>[2x]MYKTLRLGDRGADVSYLQRQLIAAGARLDIDAIYGSATRDAVMAFQATHGLVADGIAGPKTWSTLSAGRRDPRHLTDADLQRAADRLQVDLAAVRAVNEVESKGAGFLPDGRPVILYERHIMYRQLAAAGLDADALAAKYPALVNSKRGGYAGDAAEYARLASASQISGACALEATSWGAFQIMGFHWKALGYPDVFAFVDAMKVSEAEQLEAFVRFVLADKVMLAALRSKKWAKFAELYNGKAYAENLYDVKLERAFDRYSRAAA

In the present study, we describe a modular endolysin (rare for Gram-negative infecting phages) originating from B. cenocepacia AP3 phage. The structure of endolysin, predicted in silico in BLASTP, is modular, consisting of CBD (10-65 aa; PG_binding_1 domain; pfam01471) at the N-terminus, and DUF3380 domain (pfam11860) at the C-terminus (90-262 aa). Thus, comparable to lysozyme, AP3gp15 cleaves β-1,4-glycosidic bond of PG and releases GlcNAc and MurNAc. Similarly to others, the AP3 endolysin shows a broad spectrum of activity against Gram-negative strains, but no PG-degrading properties with respect to Gram-positives.

The overall structure comprises of two clearly distinguished domains, a smaller N-terminal CBD domain (Lys3 – Ser66), and a larger EAD domain (Asp77 – Ala264) located towards the C-terminus. CBD domain is composed of a bundle of three antiparallel helices (α1-α3) and is joined with EAD via a hinge region spanning amino acids (Ala67 – Thr76). The EAD domain is organized into two sub-domains: first encompassing helices α4-α5 (Asp77 – Glu101) and helices α10 to α15 (Gly185 – Ala266), and the second containing β1 (Ile115 – Tyr117), β2-β3 (Thr176 – Met184) sheet intervened by helices α6 to α9 (Arg119 – Ala175). The structure of the EAD domain of AP3gp15 is characterized by a deep concave cleft at the subdomain interface. Despite a relatively low homology of amino acid sequence (31% and 39% identity, respectively), a high structural homology of the entire AP3gp15 N-terminal part to the domains of clearly identified function strongly suggests its role in PG interaction. The large enzymatic C-terminal domain of AP3 endolysin shows structural homology to proteins of lysozyme family. The comparison to HEWL, the closest structural homologue among lysozymes, allowed to define the core structure of AP3 endolysin, where the entire fold of HEWL is encompassed within α5, α10, α12, α14 and α15. This core is decorated with large protrusions (α6-α9) characteristic only for AP3 phage endolysin and not present in classical lysozymes. The crystal structure analysis suggests that only a single catalytic residue (Glu101) is present at the active site of AP3 endolysin. Experimental data of AP3gp15 mutant Glu101Ala with a decline in activity by 99.4%, confirmed of Glu101 involvement in the catalytic reaction.>MTPEHSGRATPRWTREHASKIERTDETVVPIIYPPREDAAPEINGWDTWFLRERD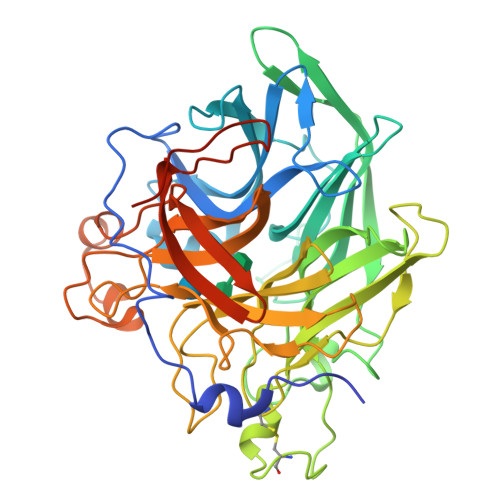GSIATVGGWRVIFSLTAPADLLPGKRHDVAEIRYFYSRDGETWFDGGPVFEGGTRGSRQWAGSALLDDDGRLYVFYTASGRAGEAEITYEQRLAVGSGGSVVADDDGVRIEGPFAHGVLLEPDGERYEREEQSRGMIYTFRDPWFFEDPRSGKTYLLFEANTPIPEGAGACGDPVWEEFNGSVGIAHSPTGDPTDWELCDPLLEGICVNQELERPHVVVRNGFYYLFVSSHDHTFAPGLEGPDGLYGFVADSLRGEYRPLNGSGLVLTNPANAPYQAYSWVAFSHREELLVSGFFNYYDLGGLTLDDVATLSPDEQRAKFGGTLAPTVRVALSGDRTRITGTLSHGRIPLESEELPDLPEERLAHREETRRGY[10x]> HHHHHHFNLPPGNYKKPVLLKSTETGQYLRINPDGTVDGTRDRSDPHIQFQISPEGNGEVLLKSTETGQYLRINPDGTVDGTRDRSDPHIQFQISPEG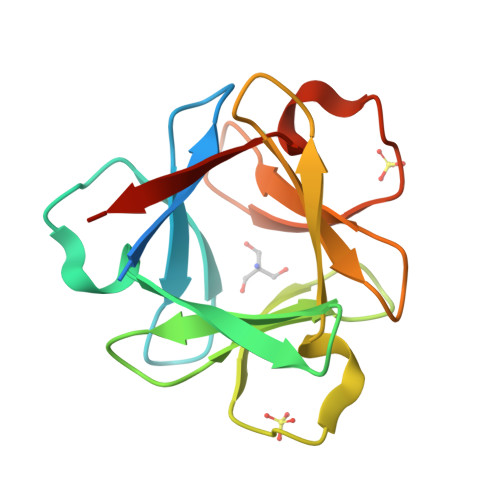NGEVLLKSTETGQYLRINPDGTVDGTRDRSDPHIQFQISPEGNG>[7x]MAEHDFETISSETLHTGA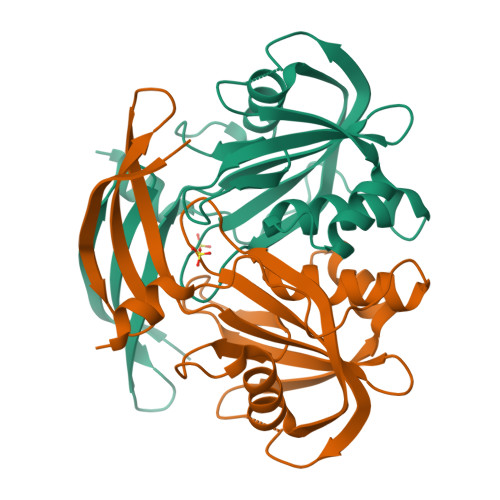IFALRRDQVRMPGGGIVTREVVEHFGAVAIVAMDDNGNIPMVYQYRHTYGRRLWELPAGLLDVAGEPPHLTAARELREEVGLQASTWQVLVDLDTAPGFSDESVRVYLATGLREVGRPEAHHEQADMTMGWYPIAEAARRVLRGEIVNSIAIAGVLAVHAVTTGFAQPRPLDTEWIDRPTAFAARRAER>SQQFNVAIFGATGAVGETMLEVLQEREFPVDELFLLASERSEGKTYRFNGKTVRVQNVEEFDWSQVHIALFSAGGELSAKWAPIAAEAGVVVIDNTSHFRYDYDIPLVVPEVNPEAIAEFRNRNIIANPNCSTIQMLVALKPIYDAVGIERINVTTYQSVSGAGKAGIDELAGQTAKLLNGYPAETNTFSQQIAFNCIPQIDQFMDNGYTKEEMKMVWETQKIFNDPSIMVNPTCVRVPVFYGHAEAVHVETRAPIDAEQVMDMLEQTDGIELFRGADFPTQVRDAGGKDHVLVGRVRNDISHHSGINLWVVADNVRK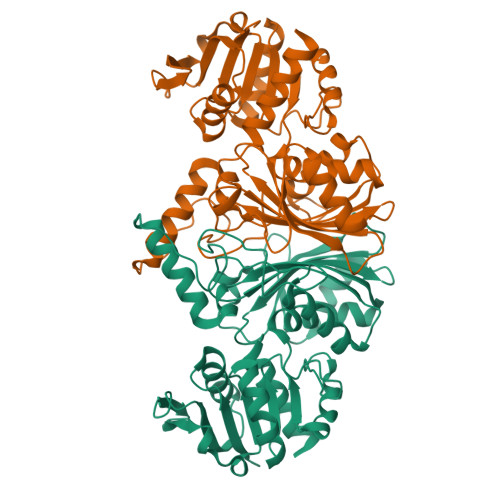GAATNAVQIAELLVRDYF[3x]> MVRLGPKKPPARKGSMADVPANLMEQIHGLETLFTVSSEKMRSIVKHFISELDKGLSKKGGNIPMIPGWVVEYPTGKETGDFLALDLGGTNLRVVLVKLGGNHDFDTTQNKYRLPDHLRTGTSEQLWSFIAKCLKEFVDEWYPDGVSEPLPLGFTFSYPASQKKINSGVLQRWTKGFDIEGVEGHDVVPMLQEQIEKLNIPINVVALINDTTGTLVASLYTDPQTKMGIIIGTGVNGAYYDVVSGIEKLEGLLPEDIGPDSPMAINCEYGSFDNEHLVLPRTKYDVIIDEESPRPGQQAFEKMTSGYYLGEIMRLVLLDLYDSGFIFKDQDISKLKEAYVMDTSYPSKIEDDPFENLEDTDDLFKTNLNIE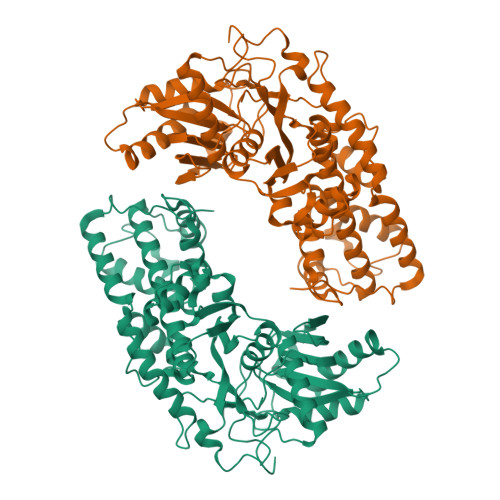TTVVERKLIRKLAELVGTRAARLTVCGVSAICDKRGYKTAHIAADGSVFNRYPGYKEKAAQALKDIYNWDVEKMEDHPIQLVAAEDGSGVGAAIIACLTQKRLAAGKSVGIKGE>[14x]MSYSGERDNFAPHMALVPMVIEQTSRGERSFDIYSRLLKERVIFLTGQVEDHMANLIVAQMLFLEAENPEKDIYLYINSPGGVITAGMSIYDTMQFIKPDVSTICMGQAASMGAFLLTAGA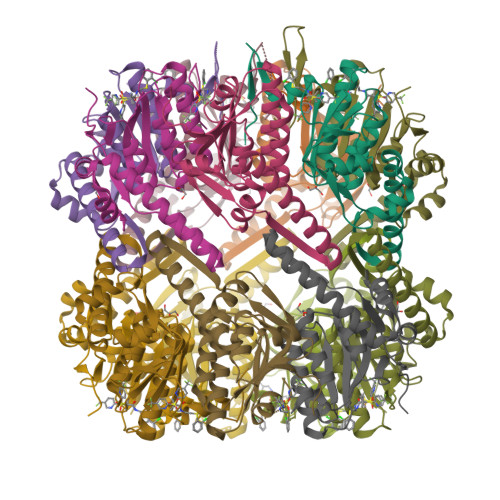KGKRFCLPNSRVMIHQPLGGYQGQATDIEIHAREILKVKGRMNELMALHTGQSLEQIERDTERDRFLSAPEAVEYGLVDSILTHRN LOVASTATIN | C24 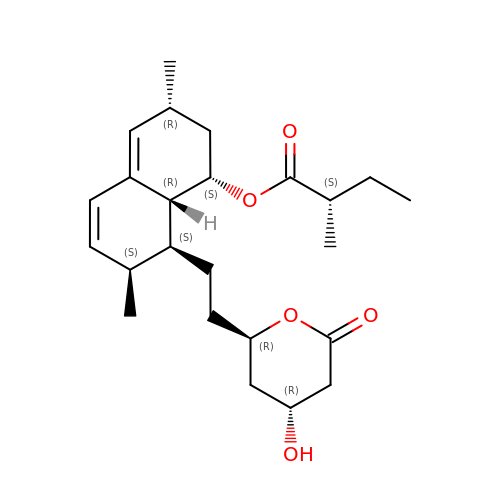H36 O5 | PCZOHLXUXFIOCF-BXMDZJJMSA-N>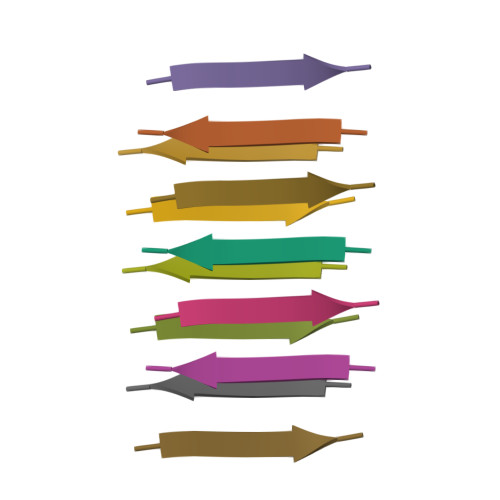AMMAAA[2x]> MVDVKKLLGKRDNSKLYEEIRKETKPKLDVNRLCRMRNDAKSDLDMWRSILQTAYHYAMPDYNPFENYGLAGFLTPGQQYNADIYDLTLPIAHKRLADKMLMNMVPQGQQWVKFTPGDEFGEPGTPLYQRALDATQRMTDHFFKIIDRSNFYLAVGESLQDVLISTGIIAINEGNRKRPVRYEAVPPAQVMFQGDAEG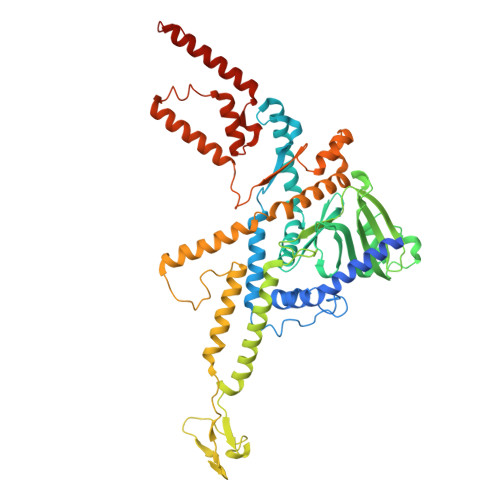QVDAIFRDWYQVRIENIKSMWPKAEVAKLNKKPEDKVDIWECAWIDYEAPEKERYQYVVMTSSKDVLLEQSNSSWPWVVYRMRRLTGEIRGRGPSLSAYPTAATINQALEDELVAAAFQANPMYMAASDSAFNQQTFTPRPGSIVPVQMVQGEWPIKPFEQSGNIQFNALLVNDFRQQINELLYAFPLGAVNSPTRTATEAEIRYTENLESFSAMVPRLQNEFFIPVIQRTLWVINKVLPETFANIPDDIRNKMISVDGQILGLSFDTPLMTAKGQVKTAALLGFYQAAASLLGPEAATASLDPVEVLTNLADNQGIDVRNIKTREELEQLLQAAGQIAQQEAAQQGVIIGSEQPQ>[2x]SNAQLGGDMKTIAIADRTGEYEQLFKENDEFRFVHAEKTAEEYRKMGADKSGIDAVLEIRQDLLEDPNAVAIYGYKQLPASVSNHISRILSDYLSDKKIASYNIPD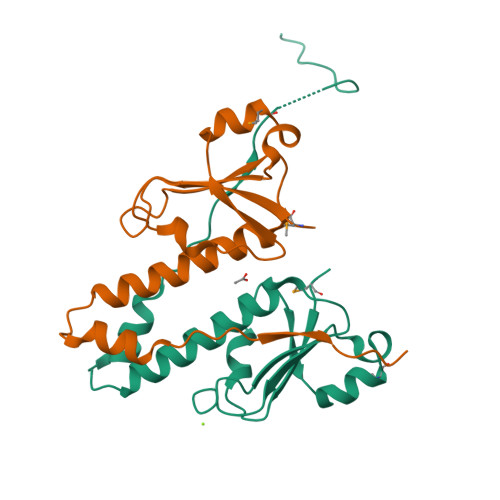IKQILADSKIELSVHTYKWSEDGTNERTSGELASGIS>VSEDLRSRIEVLKRKVIEKVQHIQLLQKNVRAQLVDMKRLEVDIDIKIRSCRGSCSRALAREVDLKDYEDQQKQLEQVIAKDLLPSR[4x];>DNENVVNEYSSELEKHQLYIDETVNSNIPTNLRVLRSILENLRSKIQKLESDVSAQMEYCRTPCTVSCNIPVVSGKECEEIIRKGGETSEMYLIQPDSSVKPYRVYCDMNTENGGWTVIQNRQDGSVDFGRKWDPYKQGFGNVATNTDGKNYCGLPGEYWLGNDKISQLTRMGPTELLIEMEDWKGDKVKAHYGGFTVQNEANKYQISVNKYRGTAGNALMDGASQLMGENRTMTIHNGMFFSTYDRDNDGWLTSDPRKQCSKEDGGGWWYNRCHAANPNGRYYWGGQYTWDMAKHGTDDGVVWMNWKGSWYSMRKMSMKIRPFFPQQ[4x];>KMLEEIMKYEASILTHDSSIRYLQEIYNSNNQKIVNLKEKVAQLEAQCQEPCKDTVQIHDITGKDCQDIANKGAKQSGLYFIKPLKANQQFLVYCEIDGSGNGWTVFQKRLDGSVDFKKNWIQYKEGFGHLSPTGTTEFWLGNEKIHLISTQSAIPYALRVELEDWNGRTSTADYAMFKVGPEADKYRLTYAYFAGGDAGDAFDGFDFGDDPSDKFFTSHNGMQFSTWDNDNDKFEGNCAEQDGSGWWMNKCHAGHLNGVYYQGGTYSKASTPNGYDNGIIWATWKTRWYSMKKTTMKIIPFNRLTIGEGQQHHLGGAK[4x];>[2x]MVWDRQRLEKELEEKKEALELAIDQASRDYHRATALEKELEEKKKALELAIDQASQDYNRANVLEKELEAITREQEINRNLLGNAKLELDQLSSEKE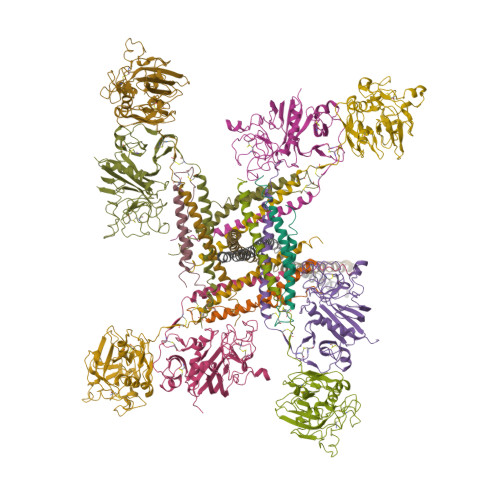QLTIEKAKLEEEKQISDASRQSLRRDLDASREAKKQVEKDLLEHHHHHH>[2x]GSSPNY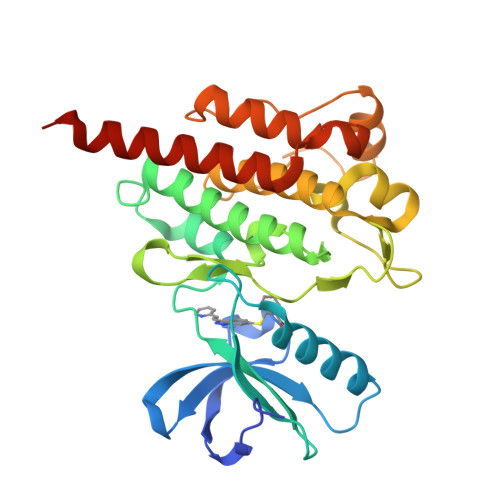DKWEMERTDITMKHKLGGGQYGEVYEGVWKKYSLTVAVKTLKEDTMEVEEFLKEAAVMKEIKHPNLVQLLGVCTREPPFYIITEFMTYGNLLDYLRECNRQEVNAVVLLYMATQISSAMEYLEKKNFIHRDLAARNCLVGENHLVKVADFGLSRLMTGDTYTAHAGAKFPIKWTAPESLAYNKFSIKSDVWAFGVLLWEIATYGMSPYPGIDLSQVYELLEKDYRMERPEGCPEKVYELMRACWQWNPSDRPSFAEIHQAFETMFQESSISDEVEKELGK>[2x]MPNSEPASLLELFNSIATQGELVRSLKAGNASKDEIDSAVKMLVSLKMSYKAAAGEDYKADCPPGNPAPTSNHGPDATEAEEDFVDPWTVQTSSAKGIDYDKLIVRFGSSKIDKELINRIERATGQRPHHFLRRGIFFSHRDMNQVLDAYENKKPFYLYTGRGPSSEAMHVGHLIPF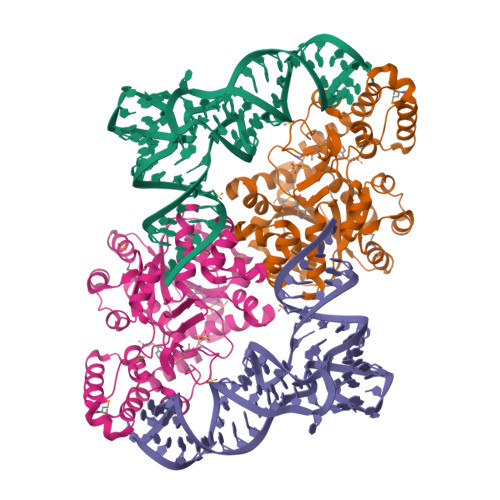IFTKWLQDVFNVPLVIQMTDDEKYLWKDLTLDQAYGDAVENAKDIIACGFDINKTFIFSDLDYMGMSSGFYKNVVKIQKHVTFNQVKGIFGFTDSDCIGKISFPAIQAAPSFSNSFPQIFRDRTDIQCLIPCAIDQDPYFRMTRDVAPRIGYPKPALLHSTFFPALQGAQTKMSASDPNSSIFLTDTAKQIKTKVNKHAFSGGRDTIEEHRQFGGNCDVDVSFMYLTFFLEDDDKLEQIRKDYTSGAMLTGELKKALIEVLQPLIAEHQARRKEVTDEIVKEFMTPRKLSFDFQHHHHHH Type-IIa receptor protein tyrosine phosphatases (RPTPs) and neurexins are the two major presynaptic organizers. In mammals, the type-IIa RPTPs have three members, PTPδ, PTPσ, and LAR. These members possess a large extracellular domain (ECD) consisting of three immunoglobulin-like (Ig) domains and four to eight fibronectin type-III (Fn) domains, followed by a single transmembrane helix and a cytoplasmic domain harboring two protein tyrosine phosphatase (PTP) domains: the first PTP domain is active, while the second domain is inactive. SALM family proteins have five isoforms (SALM1–SALM5). Their ECDs share the same domain organization consisting of a leucine-rich repeat (LRR) domain, an Ig domain and an Fn domain with 35% amino-acid sequence identity. We determined the crystal structures of apo-SALM5 (LRR–Ig), and PTPδ (Ig1–Ig3)–SALM2 (LRR–Ig) and PTPδ (Ig1–Fn1)–SALM5 (LRR–Ig) complexes at 3.08, 3.16, and 4.18 Å resolutions, respectively.

In both the PTPδ–SALM2 and PTPδ–SALM5 crystals, there are two complexes in the asymmetric unit. The binding modes of the PTPδ and SALM ECDs are quite similar between the PTPδ–SALM2 and PTPδ–SALM5 complexes: the Ig2 and Ig3 domains of PTPδ sandwiches the Ig domain of SALM2 or SALM5. The Ig2 domain of PTPδ also interacts with the LRR domain of SALM2 or SALM5. Although Pro362 of SALM5 is replaced by Ala375 in SALM2, a similar hydrogen bond is formed between the main chains of PTPδ Val143 and SALM2 Ala375 in the PTPδ–SALM2 complex. No electron density of the meA9 insert (188ESIGGTPIR196) in PTPδ Ig2 was observed in either the PTPδ–SALM2 or PTPδ–SALM5 complex, suggesting that meA is completely disordered and not involved in the binding of PTPδ to SALM2 or SALM5. The LRR domains of SALM2 and SALM5 in the asymmetric units of the crystals are aligned in an antiparallel fashion with their long sides facing each other. We therefore tested the possibility of homodimer formation of SALM2 and SALM5 LRR–Ig molecules in solution by size-exclusion chromatography coupled with multi-angle laser light scattering (SEC-MALS). The theoretical molar masses of the monomeric SALM2 and SALM5 LRR–Ig-His6 molecules are 40.2 and 41.2 kDa, whereas the molar masses of the SALM2 and SALM5 LRR–Ig-His6 molecules determined by SEC-MALS are 77.0 and 77.1 kDa, respectively, indicating that both SALM2 and SALM5 form homodimers in solution. However, we found no marked structural difference in either the PTPδ-binding or dimerization interface between the presynapse-inducing SALM5 and the non-presynapse-inducing SALM2. On the other hand, the positions of the bound PTPδ and SALM Ig relative to the SALM LRR dimers slightly differ between the PTPδ–SALM2 and PTPδ–SALM5 complexes, as shown in the superposition of these two complexes.

>LMGCVAETPPRFTRTPVDQTGVSGGVASFICQATGDPRPKIVWNKKGKKVSNQRFEVIEFDDGSGSVLRIQPLRTPRDEAIYECVASNNVGEISVSTRLTVLREDQIPRGFPTIDMGPQLKVVERTRTATMLCAASGNPDPEITWFKDFLPVDTSNNNGRIKQLRSESIGGTPIRGALQIEQSEESDQGKYECVATNSAGTRYSAPANLYVRELREVRRVPPRFSIPPTNHEIMPGGSVNITCVAVGSPMPYVKWMLGAEDLTPEDDMPIGRNVLELNDVRQSANYTCVAMSTLGVIEAIAQITVKAHHHHHH[2x];>[2x]QPCPGRCICQNVAPTLTMLCAKTGLLFVPPAIDRRVVELRLTDNFIAAVRRRDFANMTSLVHLTLSRNTIGQVAAGAFADLRALRALHLDSNRLAEVRGDQLRGLGNLRHLILGNNQIRKVESAAFDAFLSTVEDLDLSYNNLEALPWEAVGQMVNLNTLTLDHNLIDHIAEGTFVQLHKLVRLDMTSNRLHKLPPDGLFLRSQGGGPKPPTPLTVSFGGNPLHCNCELLWLRRLTREDDLETCATPEHLTDRYFWSIPEEEFLCEPPLITRQAGGRALVVEGQAVSLRCRAVGDPEPVVHWVAPDGRLLGNSSRTRVRGDGTLDVTITTLRDSGTFTCIASNAAGEATAPVEVCVVPLHHHHHH> MKLSPREIEKLGLHNAGYLAQKRLARGLRLNYTEAVALIATQIMEFVRDGDKTVAQLMSIGRELLGRRQVLPAVPKLVESVQVEATFPDGTELVTIHDPIACENGNLELALLGSFLPVPSLDKFTANDEDNRIPGEIIVVGGNLVLNDGRKAVILKVVNNGDRPVQVGSHYHFIELNPYLTFDRRKAYGMRLNIAAGNASRFEPGEMKEVLLVSIGGNKVIRGGNAIADGPVNASNCIAAMQAVITRGFGHVEEANAAEGQTG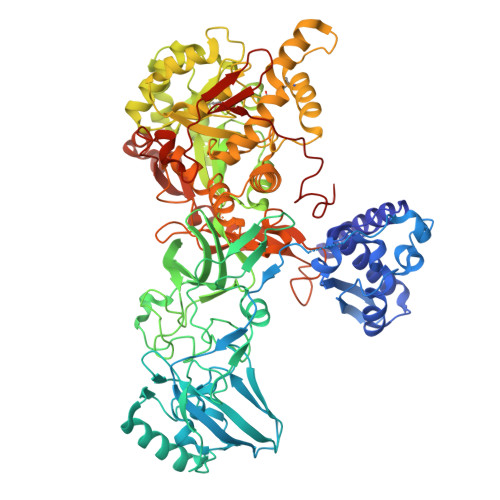EDASCPFTTVISREEYANKYGPTTGDKIRLGDTALFAEIEKDFAIYGDECTFGGGKVIRDGMGQSCGHPPALSLDTVITNAVIIDYSGIIKADIGIKDGLIHSIGKSGNPDVMDGVFQNMTTGVNTEVIAGEGLIVTAGAIDCHVHYICPQLVYEAVTSGITTLVGGGTGPTAGTRATTCTPAPIQMKLMLQSTDDLPLNFGFTGKGNCAKPDELHEIIKAGAMGLKLHEDWGTTPAAIDSCLTIAEQYDIQVNIHTDTLNESGFVEHTIAAFKGRTIHTYHSEGAGGGHAPDIIKVCGEKNVLPSSTNPTRPLTSNTIDEHVDMLMVCHHLDANIAEDVAFSASRIREATIAAEDILHDMGAISIISSDSQAMGRIGEVISRTWQTADKMKSARGPLQPGEEANDNFRIKRYVAKYTINPAIANGFSQYVGSVEVGKLADLVMWKPSFFGAKPEMVIKGGEVAYANMGDPNASIPTPEPVKMRPMYGALGKAGGALSIAFVSKAALDQRVKVLYGLNKRVEAVSNVRKLTKLDMKLNDALPAITVDPDSYTVTADGVVLTCFVATTVPLSRNYFIF>ASFETRFEKMDNLLRDPKSEVNSDCLLDGLDALVYDLDFPALRKNKNIDNFLSRYKDTINKIRDLRMKAEDYEVVKVIGRGAFGEVQLVRHKSTRKVYAMKLLSKFEMIKRSDSAFFWEERDIMAFANSPWVVQLFYAFQDDRYLYMVMEYMPGGDLVNLMSNYDVPEKWARFYTAEVVLALDAIHSMGFIHRDVKPDNMLLDKSGHLKLADFGTCMKMNKEGMVRCDTAVGTPDYISPEVLKSQGGDGYYGRECDWWSVGVFLYEMLVGDTPFYADSLVGTYSKIMNHKNSLTFPDDNDISKEAKNLICAFLTDREVR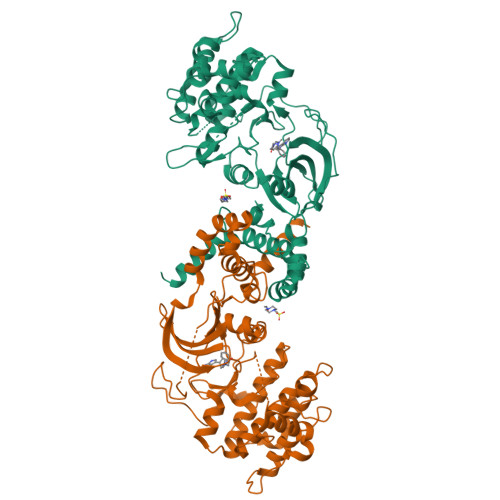LGRNGVEEIKRHLFFKNDQWAWETLRDTVAPVVPDLSSDIDTSNFDDLEEDKGEEETFPIPKAFVGNQLPFVGFTYYSN[4x]> GSSDKGKLSLQDVAELIRARACQRVVVMVGAGISTPSGIPDFRSPGSGLYSNLQQYDLPYPEAIFELPFFFHNPKPFF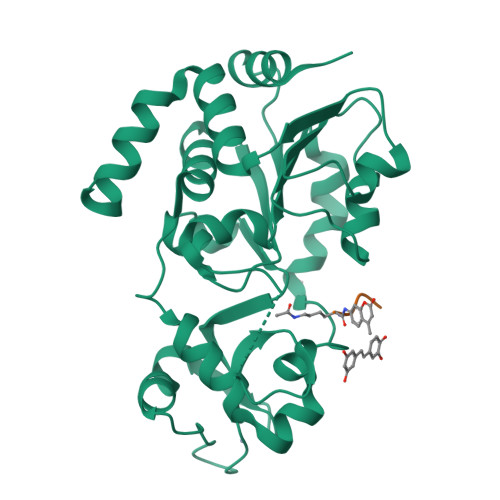TLAKELYPGNYKPNVTHYFLRLLHDKGLLLRLYTQNIDGLERVSGIPASKLVEAHGTFASATCTVCQRPFPGEDIRADVMADRVPRCPVCTGVVKPDIVFFGEPLPQRFLLHVVDFPMADLLLILGTSLEVEPFASLTEAVRSSVPRLLINRDLVGPLAWHPRSRDVAQLGDVVHGVESLVELLGWTEEMRDLVQRETGKLDGPDK>MKPEVEQELAHILLTELLAYQFASPVRWIETQDVFLKDFNTERVVEIGPSPTLAGMAQRTLKNKYESYDAALSLHREILCYSKDAKEIYYTPDPSELAAKEEPAKEEAPAPTPAASAPAPAAAAPAPVAAAAPAAAAAEIADEPVKASLLLHVLVAHKLKKSLDSIPMSKTIKDLVGGKSTVQNEILGDLGKEFGTTPEKPEETPLEELAETFQDTFSGALGKQSSSLLSRLISSKMPGGFTITVARKYLQTRWGLPSGRQDGVLLVALSNEPAARLGSEADAKAFLDSMAQKYASIVGVDLSSAASASGAAGAGAAAGAAMIDAGALEEITKDHKVLARQQLQVLARYLKMDLDNGERKFLKEKDTVAELQAQLDYLNAELGEFFVNGVATSFSRKKARTFDSSWNWAKQSLLSLYFEIIHGVLKNVDREVVSEAINIMNRSNDALIKFMEYHISNTDETKGENYQLVKTLGEQLIENCKQVLDVDPVYKDVAKPTGPKTAIDKNGNITYSEEPREKVRKLSQYVQEMALGGPITKESQPTIEEDLTRVYKAISAQADKQDISSSTRVEFEKLYSDLMKFLESSKEIDPSQTTQLAGMDVEDALDKDSTKEVASLPNKSTISKTVSSTIPRETIPFLHLRKKTPAGDWKYDRQLSSLFLDGLEKAAFNGVTFKDKYVLITGAGKGSIGAEVLQGLLQGGAKVVVTTSRFSKQVTDYYQSIYAKYGAKGSTLIVVPFNQGSKQDVEALIEFIYDTEKNGGLGWDLDAIIPFAAIPEQGIELEHIDSKSEFAHRIMLTNILRMMGCVKKQKSARGIETRPAQVILPMSPNHGTFGGDGMYSESKLSLETLFNRWHSESWANQLTVCGAIIGWTRGTGLMSANNIIAEGIEKMGVRTFSQKEMAFNLLGLLTPEVVELCQKSPVMADLNGGLQFVPELKEFTAKLRKELVETSEVRKAVSIETALEHKVVNGNSADAAYAQVEIQPRANIQLDFPELKPYKQVKQIAPAELEGLLDLERVIVVTGFAEVGPWGSARTRWEMEAFGEFSLEGCVEMAWIMGFISYHNGNLKGRPYTGWVDSKTKEPVDDKDVKAKYETSILEHSGIRLIEPELFNGYNPEKKEMIQEVIVEEDLEPFEASKETAEQFKHQHGDKVDIFEIPETGEYSVKLLKGATLYIPKALRFDRLVAGQIPTGWNAKTYGISDDIISQVDPITLFVLVSVVEAFIASGITDPYEMYKYVHVSEVGNCSGSGMGGVSALRGMFKDRFKDEPVQNDILQESFINTMSAWVNMLLISSSGPIKTPVGACATSVESVDIGVETILSGKARICIVGGYDDFQEEGSFEFGNMKATSNTLEEFEHGRTPAEMSRPATTTRNGFMEAQGAGIQIIMQADLALKMGVPIYGIVAMAATATDKIGRSVPAPGKGILTTAREHHSSVKYASPNLNMKYRKRQLVTREAQIKDWVENELEALKLEAEEIPSEDQNEFLLERTREIHNEAESQLRAAQQQWGNDFYKRDPRIAPLRGALATYGLTIDDLGVASFHGTSTKANDKNESATINEM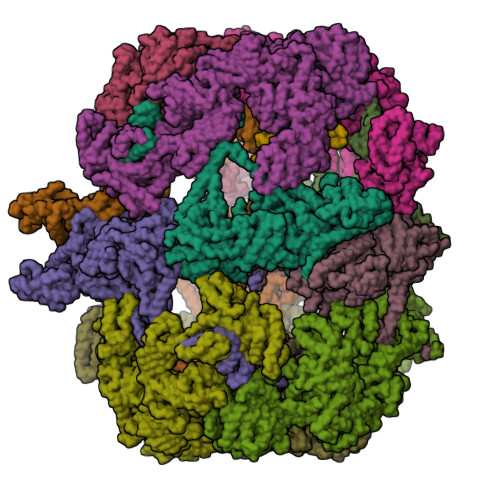MKHLGRSEGNPVIGVFQKFLTGHPKGAAGAWMMNGALQILNSGIIPGNRNADNVDKILEQFEYVLYPSKTLKTDGVRAVSITSFGFGQKGGQAIVVHPDYLYGAITEDRYNEYVAKVSAREKSAYKFFHNGMIYNKLFVSKEHAPYTDELEEDVYLDPLARVSKDKKSGSLTFNSKNIQSKDSYINANTIETAKMIENMTKEKVSNGGVGVDVELITSINVENDTFIERNFTPQEIEYCSAQPSVQSSFAGTWSAKEAVFKSLGVKSLGGGAALKDIEIVRVNKNAPAVELHGNAKKAAEEAGVTDVKVSISHDDLQAVAVAVSTKK[12x];>MDAYSTRPLTLSHGSLEHVLLVPTASFFIASQLQEQFNKILPEPTEGFAADDEPTTPAELVGKFLGYVSSLVEPSKVGQFDQVLNLCLTEFENCYLEGNDIHALAAKLLQENDTTLVKTKELIKNYITARIMAKRPFDKKSNSALFRAVGEGNAQLVAIFGGQGNTDDYFEELRDLYQTYHVLVGDLIKFSAETLSELIRTTLDAEKVFTQGLNILEWLENPSNTPDKDYLLSIPISCPLIGVIQLAHYVVTAKLLGFTPGELRSYLKGATGHSQGLVTAVAIAETDSWESFFVSVRKAITVLFFIGVRCYEAYPNTSLPPSILEDSLENNEGVPSPMLSISNLTQEQVQDYVNKTNSHLPAGKQVEISLVNGAKNLVVSGPPQSLYGLNLTLRKAKAPSGLDQSRIPFSERKLKFSNRFLPVASPFHSHLLVPASDLINKDLVKNNVSFNAKDIQIPVYDTFDGSDLRVLSGSISERIVDCIIRLPVKWETTTQFKATHILDFGPGGASGLGVLTHRNKDGTGVRVIVAGTLDINPDDDYGFKQEIFDVTSNGLKKNPNWLEEYHPKLIKNKSGKIFVETKFSKLIGRPPLLVPGMTPCTVSPDFVAATTNAGYTIELAGGGYFSAAGMTAAIDSVVSQIEKGSTFGINLIYVNPFMLQWGIPLIKELRSKGYPIQFLTIGAGVPSLEVASEYIETLGLKYLGLKPGSIDAISQVINIAKAHPNFPIALQWTGGRGGGHHSFEDAHTPMLQMYSKIRRHPNIMLIFGSGFGSADDTYPYLTGEWSTKFDYPPMPFDGFLFGSRVMIAKEVKTSPDAKKCIAACTGVPDDKWEQTYKKPTGGIVTVRSEMGEPIHKIATRGVMLWKEFDETIFNLPKNKLVPTLEAKRDYIISRLNADFQKPWFATVNGQARDLATMTYEEVAKRLVELMFIRSTNSWFDVTWRTFTGDFLRRVEERFTKSKTLSLIQSYSLLDKPDEAIEKVFNAYPAAREQFLNAQDIDHFLSMCQNPMQKPVPFVPVLDRRFEIFFKKDSLWQSEHLEAVVDQDVQRTCILHGPVAAQFTKVIDEPIKSIMDGIHDGHIKKLLHQYYGDDESKIPAVEYFGGESPVDVQSQVDSSSVSEDSAVFKATSSTDEESWFKALAGSEINWRHASFLCSFITQDKMFVSNPIRKVFKPSQGMVVEISNGNTSSKTVVTLSEPVQGELKPTVILKLLKENIIQMEMIENRTMDGKPVSLPLLYNFNPDNGFAPISEVMEDRNQRIKEMYWKLWIDEPFNLDFDPRDVIKGKDFEITAKEVYDFTHAVGNNCEDFVSRPDRTMLAPMDFAIVVGWRAIIKAIFPNTVDGDLLKLVHLSNGYKMIPGAKPLQVGDVVSTTAVIESVVNQPTGKIVDVVGTLSRNGKPVMEVTSSFFYRGNYTDFENTFQKTVEPVYQMHIKTSKDIAVLRSKEWFQLDDEDFDLLNKTLTFETETEVTFKNANIFSSVKCFGPIKVELPTKETVEIGIVDYEAGASHGNPVVDFLKRNGSTLEQKVNLENPIPIAVLDSYTPSTNEPYARVSGDLNPIHVSRHFASYANLPGTITHGMFSSASVRALIENWAADSVSSRVRGYTCQFVDMVLPNTALKTSIQHVGMINGRKLIKFETRNEDDVVVLTGEAEIEQPVTTFVFTGQGSQEQGMGMDLYKTSKAAQDVWNRADNHFKDTYGFSILDIVINNPVNLTIHFGGEKGKRIRENYSAMIFETIVDGKLKTEKIFKEINEHSTSYTFRSEKGLLSATQFTQPALTLMEKAAFEDLKSKGLIPADATFAGHSLGEYAALASLADVMSIESLVEVVFYRGMTMQVAVPRDELGRSNYGMIAINPGRVAASFSQEALQYVVERVGKRTGWLVEIVNYNVENQQYVAAGDLRALDTVTNVLNFIKLQKIDIIELQKSLSLEEVEGHLFEIIDEASKKSAVKPRPLKLERGFACIPLVGISVPFHSTYLMNGVKPFKSFLKKNIIKENVKVARLAGKYIPNLTAKPFQVTKEYFQDVYDLTGSEPIKEIIDNWEKYEQS[12x];>MCSAGGIRRPIQIEEFKTAISGMSDMELAQIKTEIENSINHLQRSNARLGKYIAKLEGADDRLEADDSDDLENIDSGDLALYKDSVRENEIVLNNYNERVDALEQETVYRKTGHGKSKHEVEAKDNTNKGPDVDMDNSNVDVVTPNSIFI[12x]> EHVRRDLDPNEVWEIVGELGDGAFGKVYKAKNKETGALAAAKVIETKSEEELEDYIVEIEILATCDHPYIVKLLGAYYHDGKLWIMIEFCPGGAVD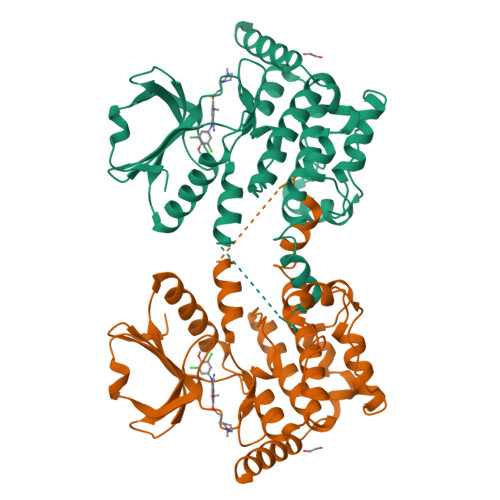AIMLELDRGLTEPQIQVVCRQMLEALNFLHSKRIIHRDLKAGNVLMTLEGDIRLADFGVSAKNLKTLQKRDSFIGTPYWMAPEVVMCETMKDTPYDYKADIWSLGITLIEMAQIEPPHHELNPMRVLLKIAKSDPPTLLTPSKWSVEFRDFLKIALDKNPETRPSAAQLLEHPFVSSITSNKALRELVAEAKAEVME>MHHHHHHSNNNTSIHDFDFSFICNYFKLLKRQGPGSPEATRKAVSFINELTDDAKIADIGCGTGGQTLFLADYVKGQITGIDLFPDFIEIFNENAVKANCADRVKGITGSMDNLPFQNEELDLIWSEGAIYNIGFERGMNEWS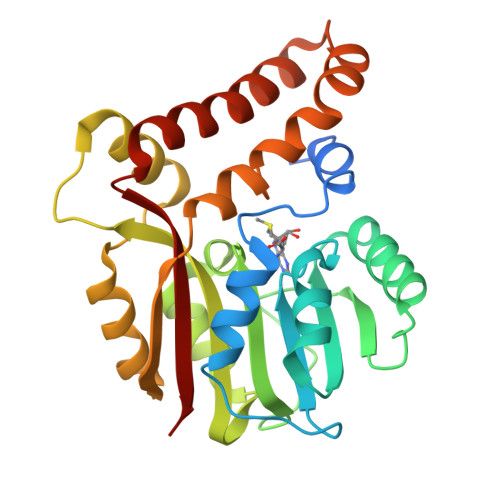KYLKKGGFIAVSEASWFTSERPAEIEDFWMDAYPEISVIPTCIDKMERAGYTPTAHFILPENCWTEHYFAPQDEVRETFMKEHAGNKTAMDFMKGQQYERSLYSKYKDYYGYVFYIGQKR[2x]(3~{S})-6'-azanyl-7-fluoranyl-2,2,3'-trimethyl-5-pyridin-4-yl-spiro[1~{H}-indene-3,4'-2~{H}-pyrano[2,3-c]pyrazole]-5'-carbonitrile 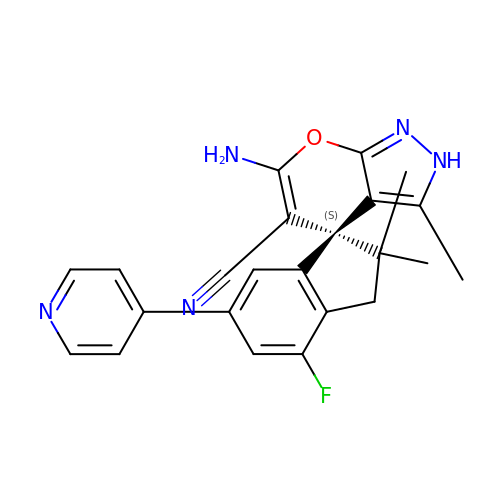| C23 H20 F N5 O | QSHPRVNBDFMPTJ-HSZRJFAPSA-N In plants, DNA methylation occurs in CG, CHG, and CHH contexts (where H = A, T, or C), with the maintenance of CG methylation mediated by the DNA methyltransferase MET1. MET1 possesses replication foci target sequence (RFTS) 1–2, acidic-linker, bromo adjacent homology (BAH) 1–2 and methyltransferase (MTase) domains, whereas DNMT1 possesses PCNA-binding, RFTS, CXXC, autoinhibitory linker, BAH1-2 and MTase domains. Of note, MET1 has two RFTS domains and lacks the CXXC domain. Arabidopsis thaliana MET1 exhibits a plant-specific structural feature in the autoinhibition state, and a conserved activation state compared to mammalian DNMT1.

Cryo-EM map of apo-MET1full was reconstructed at 3.21 Å resolution; the RFTS1 domain (aa: 1–345), the acidic-linker (aa: 648–707), loops in the BAH2 domain (aa: 926–934 and 958–965) and the catalytic loop in the MTase domain were completely disordered reflecting a highly flexible state. The domain assembly of the core region of apo-MET1full, BAH1–BAH2–MTase, was identical to that of MET1MTase bound to the hemimethylated DNA complex with an RMSD of 0.550 Å over 776 aligned Cα atoms. The structure of apo-MET1full revealed that the RFTS2 domain contacted the TRD in the MTase domain and residues 601–610 in the connecting linker (aa: 599–623) between the RFTS2 domain and the Activating Helix, contributing to the stable spatial position of the RFTS2 domain (e left). This spatial positioning of the RFTS2 domain caused a severe steric clash with hemimethylated DNA, in which residues 360–366 and 397–405 of the N-lobe in the RFTS2 domain played a potential inhibitory role in DNA-binding when compared to the DNA bound form of MET1. Intriguingly, the connecting linker was rigidly positioned across the axis of the DNA duplex bound to the catalytic core, suggesting that the connecting linker reinforces the autoinhibitory state of apo-MET1full. In the structure of apo-MET1full, the DNA Recognition Helix (aa:1208–1231) in the MTase domain was kinked at Met1219, resulting in disorder of the subsequent catalytic loop, in which the Toggle Pocket composed of Ile1220, Phe1235, Phe1246, Thr1251, and Leu1254 of the MTase domain accepted side chain of Val1215 of the DNA Recognition Helix. The Activating Helix of apo-MET1full formed a three-turn helical conformation, which differed from the turn conformation following the two-turn helix of MET1MTase bound to the DNA complex. In clear contrast, the RFTS2 domain of MET1 was positioned in an upside-down orientation and the N-lobe of the RFTS2 domain was associated with the TRD in the MTase domain away from the DNA binding pocket. Asp402, Asp420, and Asn422 of the N-lobe in the RFTS2 domain formed hydrogen bonds with Arg1393, Lys1412, and Val1420 of TRD, respectively, resulting in spatially different position from that of the RFTS domain in DNMT1.

> GPPTTMVENGAKAAKRKKRPLPEIQEVEDVPRTRRPRRAAACTSFKEKSIRVCEKSATIEVKKQQIVEEEFLALRLTALETDVEDRPTRRLNDFVLFDSDGVPQPLEMLEIHDIFVSGAILPSDVCTDKEKEKGVRCTSFGRVEHWSISGYEDGSPVIWISTELADYDCRKPAASYRKVYDYFYEKARASVAVYKKLSKSSGGDPDIGLEELLAAVVRSMSSGSKYFSSGAAIIDFVISQGDFIYNQLAGLDETAKKHESSYVEIPVLVALREKSSKIDKPLQRERNPSNGVRIKEVSQVAESEALTSDQLVDGTDDDRRYAILLQDEENRKSMQQPRKNSSSGSASNMFYIKINEDEIANDYPLPSYYKTSEEETDELILYDASYEVQSEHLPHRMLHNWALYNSDLRFISLELLPMKQCDDIDVNIFGSGVVTDDNGSWISLNDPDSGSQSHDPDGMCIFLSQIKEWMIEFGSDDIISISIRTDVAWYRLGKPSKLYAPWWKPVLKTARVGISILTFLRVESRVARLSFADVTKRLSGLQANDKAYISSDPLAVERYLVVHGQIILQLFAVYPDDNVKRCPFVVGLASKLEDRHHTKWIIKKKKISLKELNLNPRAGMAPVASKRKAMQATTTRLVNRIWGEFYSNYSPEDPLQATAAENGEDEVEEEGGNGEEEVEEEGENGLTEDTVPEPVEVQKPHTPKKIRGSSGKREIKWDGESLGKTSAGEPLYQQALVGGEMVAVGGAVTLEVDDPDEMPAIYFVEYMFESTDHCKMLHGRFLQRGSMTVLGNAANERELFLTNECMTTQLKDIKGVASFEIRSRPWGHQYRKKNITADKLDWARALERKVKDLPTEYYCKSLYSPERGGFFSLPLSDIGRSSGFCTSCKIREDEEKRSTIKLNVSKTGFFINGIEYSVEDFVYVNPDSIGGLKEGSKTSFKSGRNIGLRAYVVCQLLEIVPKESRKADLGSFDVKVRRFYRPEDVSAEKAYASDIQELYFSQDTVVLPPGALEGKCEVRKKSDMPLSREYPISDHIFFCDLFFDTSKGSLKQLPANMKPKFSTIKDDTLLRKKKGKGVESEIESEIVKPVEPPKEIRLATLDIFAGCGGLSHGLKKAGVSDAKWAIEYEEPAGQAFKQNHPESTVFVDNCNVILRAIMEKGGDQDDCVSTTEANELAAKLTEEQKSTLPLPGQVDFINGGPPCQGFSGMNRFNQSSWSKVQCEMILAFLSFADYFRPRYFLLENVRTFVSFNKGQTFQLTLASLLEMGYQVRFGILEAGAYGVSQSRKRAFIWAAAPEEVLPEWPEPMHVFGVPKLKISLSQGLHYAAVRSTALGAPFRPITVRDTIGDLPSVENGDSRTNKEYKEVAVSWFQKEIRGNTIALTDHICKAMNELNLIRCKLIPTRPGADWHDLPKRKVTLSDGRVEEMIPFCLPNTAERHNGWKGLYGRLDWQGNFPTSVTDPQPMGKVGMCFHPEQHRILTVRECARSQGFPDSYEFAGNINHKHRQIGNAVPPPLAFALGRKLKEALHLKKSPQHQP> GMNSLLSRALELQRMAHELMYLDTNGSPIYSDEFCRLNKEVLTRSDSLFSEQSSDIEEEG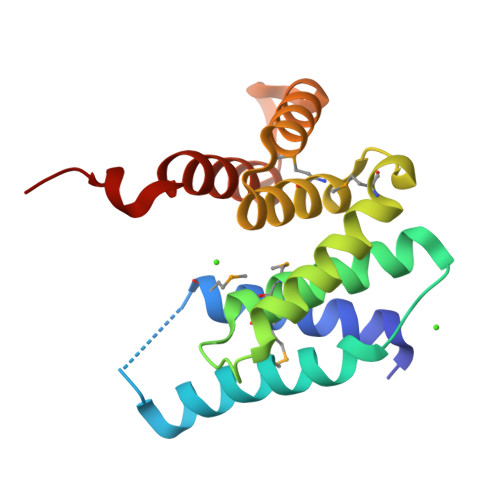NLCLALLMGYNATIYDNGDKERKKQVILDRIYNIMSQLPASLLKMRLLTWGYSETYDEELAHEAHQLIETWNISDLTDEQKEIIEELRNFEENQYPWEEVQE>AMEQLLRAELRTATLRAFGGPGAGCISEGRAYDTDAGPVFVKVNRRTQARQMFEGEVASLEALRSTGLVRVPRPMKVIDLPGGGAAFVMEHLKMKSLSSQASKLGEQMADLHLYNQKGSSYVDKFGFHTVTCCGFIPQVNEWQDDWPTFFARHRLQAQLDLIEKDYADREARELWSRLQVKIPDLFCGLEIVPALLHGDLWSGNVAEDDVGPIIYDPASFYGHSEFELAIALMFGGFPRSFFTAYHRKIPK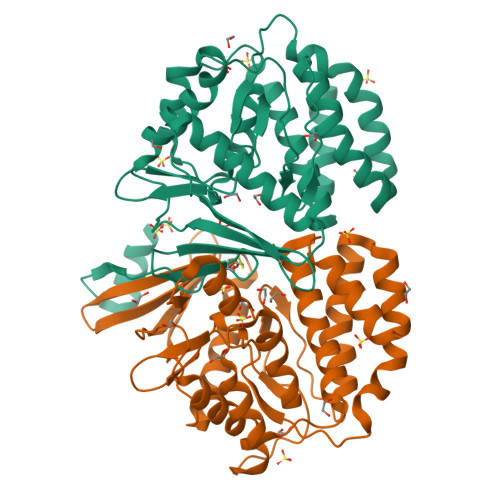APGFDQRLLLYQLFNYLNHWNHFGREYRSPSLGTMRRLLK[2x]>MKKLLALGLLGLVLASCGKKEETTTGPKETTIFAMHLGKALDPNLPVFVKAEKDTNIKLVNVASQNQTDQIQAYNLMLTEGKLPDIVSYELSADLENLGIEGGLIPLEDLINQHAPNLKKFFEENPRYKKDAVAVDGHIYMIPNYYDYFNIKVSQGYFIRQDWLEKLGLKEPRTVDELYTTLKAFREKDPNGNGKKDEVPFFVRANNVRKVLTSLVDLFKASPIWYEENGMVKYGPAQKEFKHAIKELSKWYKEGLIDEEIFTRGLESRDYLLSNNLGGATDDWIASTSSYNRNLADKIPGFNLKLVLPYELNGNAKTRHARTTYLGGWGISKDAKDPVSLIKYFDYWYSVEGRRLWNFGIEGSEYTLVDGKPVFTDKVLKNPDGKTPLAVLREVGAQYRLGAFQDAQYELGWASESAKAGYKYYMDNDVVLDELPILKYTKEKSKEFVSIDTAMRAVVEEKAQQWILGSGDIDKEWDAYIKRLENLGLSKAEQIQNEAFKNFNK[4x]

The solute-binding protein (Smon0123) captures GAG disaccharides in the periplasm and delivers them to the ABC transporter, followed by their import in the cytoplasm. The ABC transporter comprises membrane-spanning proteins (Smon0121-Smon0122) as heterodimers and ATPase domains (Smon0120-Smon0120) as homodimers. Similar to other solute-binding proteins, Smon0123 has two major N and C domains that are connected via a flexible hinge and that captures the substrates via a mechanism called the “Venus’s flytrap”. Because of a large molecular size (57 kDa) and EF hand-like calcium-binding site, Smon0123 should also be added to the 7th cluster.

The purified Smon0123 (N-18/C-5) was crystallized in the presence of CΔ4S6S, and the resultant crystal was suitable for determining the structure. The refined model contained four monomers in an asymmetric unit while the biological unit was monomer. In the complex crystal structure of Smon0123 with CΔ4S6S, the substrate CΔ4S6S was bound to a cleft between the N and C domains. Far from the cleft, a calcium ion was bound to the C1 subdomain. Two positively charged residues, Arg204 and Arg393, were directly bound to the sulfate group at the C-4 position. Lys210 directly formed hydrogen bonds with the sulfate group at the C-6 position. Moreover, aromatic residues such as Tyr146 and Trp284 interacted with the pyranose ring of the substrate. On the other hand, the magnitude of the hinge-bending motion of the Smon0123/CΔ4S6S structure was determined to be 39°. Therefore, two sulfate groups in CΔ4S6S shifted the arrangements of amino acid residues in the C1 subdomain, resulting in conformational changes in Smon0123/CΔ4S6S owing to the movement of the C domain. As a result, the enhancement of its ATPase activity in the presence of CΔ4S6S was lower than that of CΔ0S and CΔ4S, suggesting that CΔ4S6S-bound Smon0123 in the 39°-closed conformation is unpreferable for docking with the ABC transporter compared to that in the 47°-closed conformation.> MAVTYEKTFEIEIINELSASVYNRVLNYVLNHELNKNDSQLLEVNLLNQLKLAKRVNLFDYSLEELQ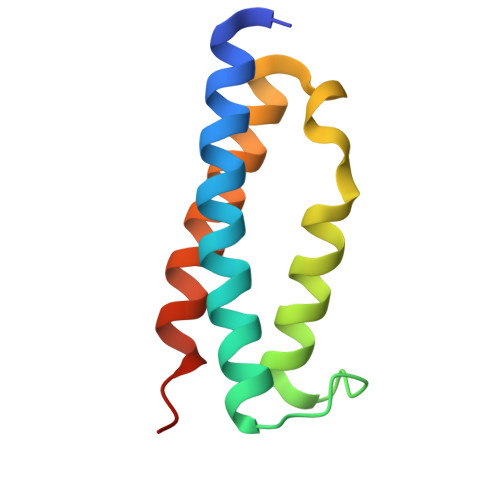AVHEYWRSMNRYSKQVLNKEKVA(1R)-1-(1-cyclopentyl-1H-pyrazol-4-yl)ethan-1-ol | C10 H16 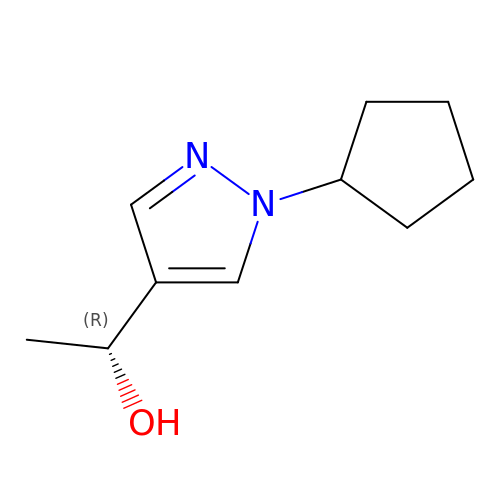N2 O | TUZCKTQECDPISK-UHFFFAOYSA-N>PPTIHRNLLSPELVQWALKIEKDSRLTARGALAVMSYAKTGRSPLDKRIVDTDDVRENVDWGKVNMKLSEESFARVRKIAKEFLDTREHLFVVDCFAGHDERYRLKVRVFTTRPYHALFMRDMLIV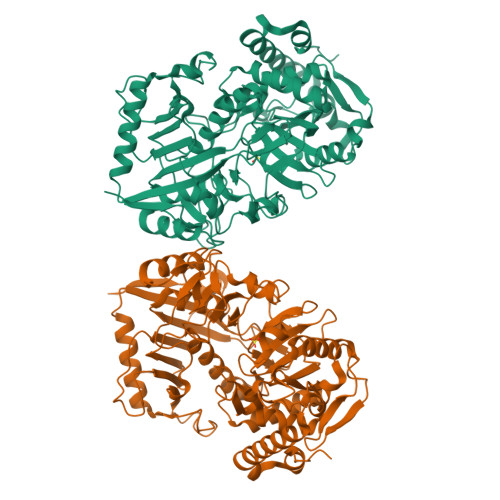PTPEELATFGEPDYVIYNAGECKADPSIPGLTSTTCVALNFKTREQVILGTEYAGEMKKGILTVMFELMPQMNHLCMHASANVGKQGDVTVFFGLSGTGKTTLSADPHRNLIGDDEHVWTDRGVFNIEGGCYAKAIGLNPKTEKDIYDAVRFGAVAENCVLDKRTGEIDFYDESICKNTRVAYPLSHIEGALSKAIAGHPKNVIFLTNDAFGVMPPVARLTSAQAMFWFVMGYTANVPGVEAGGTRTARPIFSSCFGGPFLVRHATFYGEQLAEKMQKHNSRVWLLNTGYAGGRADRGAKRMPLRVTRAIIDAIHDGTLDRTEYEEYPGWGLHIPKYVAKVPEHLLNPRKAWKDVRQFNETSKELVAMFQESFSARFAAKASQEMKSAVPRYVEFARL[2x]[4-(4-amino-6,7-dimethoxyquinazolin-2-yl)piperazin-1-yl][(2R)-tetrahydrofuran-2-yl]methanone | 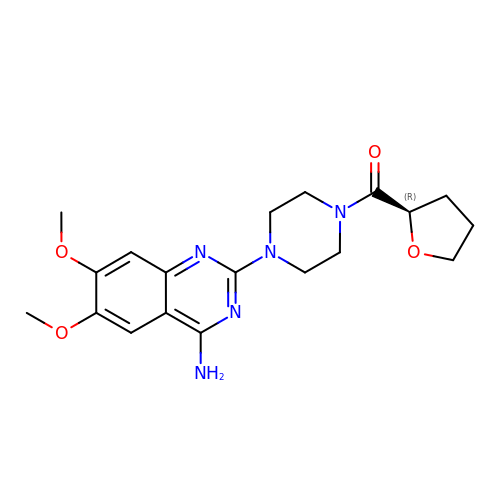C19 H25 N5 O4 | VCKUSRYTPJJLNI-CQSZACIVSA-N>GLRRLTIRDLLAQGRTSSNALEYVREEVFTNNADVVAEKALKPESDITFSKQTANVKTIAHWVQASRQVMDDAPMLQSYINNRLMYGLALKEEGQLLNGDGTGDNLEGLNKVATAYDTSLNATGDTRADIIAHAIYQVTESEFSASGIVLNPRDWHNIALLKDNEGRYIFGGPQAFTSNIMWGLPVVPTKAQAAGTFTVGGFDMASQVWDRMDATVEVSREDRDNFVKNMLTILCEERLALAHYRPTAIIK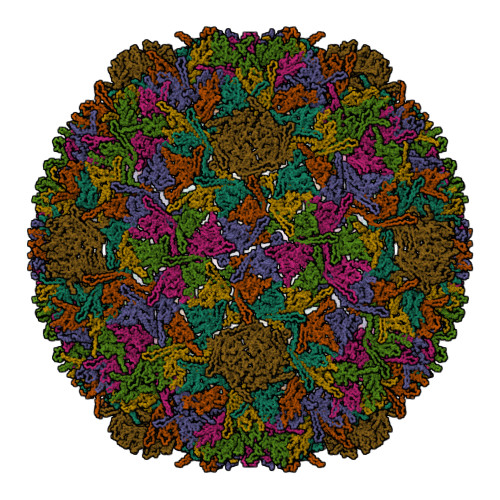GTFSS[7x]> GSAGEDVGAPPDHLWVHQEGIYRDEYQRTWVAVV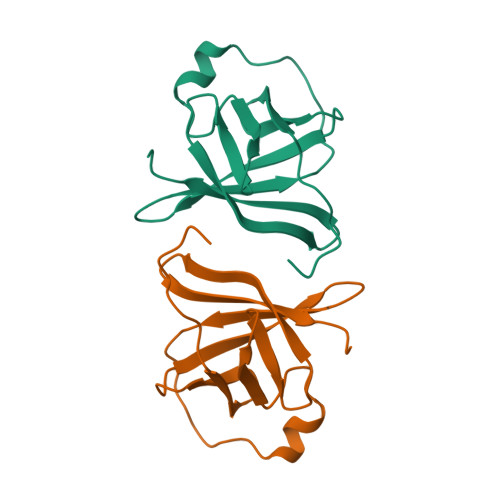EEETSFLRARVQQIQVPLGDAARPSHLLTSQLPLMWQLYPEERYMDNNSRLWQIQHHLMVRGVQELLLKLLPDD> MASSYSASAEPARVRALVYGHHGDPAKVVELKNLELAAVRGSDVRVKMLAAPINPSDINMIQGNYGLLPELPAVGGNEGVAQVVAVGSNVTGLKPGDWVIPANAGLGTWRTEAVFSEEALIQVPSDIPLQSAATLGVNPCTAYRMLMDFEQLQPGDSVIQNASNSGVGQAVIQIAAALGLRTINVVRDRPDIQKLSDRLKSLGAEHVITEEELRRPEMKNFFKDMPQPRLALNCVGGKSSTELLRQLARGGTMVTYGGMAKQPVVASVSLLIFKDLKLRGFWLSQWKKDHSPDQFKELILTLCDLIRRGQLTAPACSQVPLQDYQSALEASMKPFISSKQILTMLEHHHHHH

Mitochondrial fatty acid synthesis (mtFAS) is essential for respiratory function. The last step of mtFAS is carried out by 2E-enoyl-ACP thioester reductases MECR and Etr1 in human and yeast, respectively. These enzymes are members of the medium-chain dehydrogenase / reductase (MDR) superfamily, catalyzing the NADPH-dependent reduction of 2E-enoyl thioesters into acyl thioesters. The structure of MECR shows a bent cavity of sufficient dimensions to accommodate acyl substrates with carbon chain lengths from C4 to C1619.

G165Q variant did not provide crystals under conditions previously used in MECR crystallization, so completely new crystallization parameters were screened. Both wild-type and the G165Q MECR formed hexagonal crystals at +4 °C in a condition where the main precipitation agents were PEG 6000 and NaCl and the pH was 4.5 as described in Material and Methods. Crystal structures were solved at 1.85 Å and 2.02 Å resolution, respectively, in the trigonal space group P3121. The asymmetric unit contains one MECR chain, but the enzyme forms a dimer via a crystallographic 2-fold axis. In the MECR structures presented here, the first N-terminal residues (residues A31-A41) are not defined by the electron density maps, but the C-terminus (till L374) including the six residue long His-tag sequence is seen well. Otherwise, the current and previous wild-type structures are very similar (RMSD 0.70 Å for 332 aligned residues). There are some small differences in certain loop regions such as 240-252. In the current structure this region has high B factors, but residues are still well defined by the electron density maps. In the wild-type MECR, the substrate binding cavity can accommodate fatty acyl substrate longer than C8.The aromatic ring system of these compounds is able to include lysine and arginine side chains, supported by one or two phosphate groups that are attached to the half-moon-shaped molecule. Furthermore, we solved crystal structures of two different tweezer variants in complex with the enzyme Δ1-Pyrroline-5-carboxyl-dehydrogenase (P5CDH) and found that the tweezers are bound to a lysine and methionine side chain, respectively. Therefore, P5CDH was chosen as a target for the systematic analysis of co-crystallization with two different tweezer molecules, the diphosphate tweezer CLR01, which was also used for the 14-3-3 structures, and a monophosphate tweezer, where one phosphate group is replaced by a sterically less-demanding hydroxyl group. In both crystals, only one tweezer molecule is seen in the asymmetric unit despite the presence of two and four monomers of P5CDH, respectively, revealing an asymmetric binding mode of the tweezer to P5CDH, depending on the non-equivalent environment of the tweezer binding sites in the monomers.

P5CDH crystallizes as a tetramer consisting of a dimer of the physiologically relevant dimers with the N-termini of all four molecules in the asymmetric unit packing together in a large cleft between the two dimers formed by chains A and B, or C and D, respectively. Surprisingly, the CLR01 molecule was found in only one copy per tetramer in the asymmetric unit, and instead of binding to a lysine or arginine side chain, as expected, the Met17 of chain A—which actually belongs to artificially introduced linker residues —was seen as the guest inside the aromatic ring. The tweezer bound to monomer A is stabilized by packing against residues of monomer D. Interestingly, the regions around Met17 in monomers B, C, and D are disordered, indicating that the binding of CLR01 has a stabilizing effect on the N-terminus of monomer A, similar to the effect on the binding of a peptide to 14-3-3 described in the previous section. To further validate this binding mode, the anomalous signal of phosphorous and sulfur was measured at a wavelength of 1.698 Å at the synchrotron. Three peaks are observed at 2I/σI, at both phosphate groups of the tweezer and inside the ring system at a position corresponding to the sulfur atom of methionine 17. Although the anomalous signal is relatively weak, this strongly supports the binding mode of the tweezer encircling the Met17 side chain. A more detailed analysis of the tweezer binding modes using the CCP4 PISA software revealed that the largest hydrophobic Van der Waals interactions between the CLR01 and P5CDH monomer A are from the Met17 side chain bound inside the aromatic ring system, which is additionally clamped between two lysine residues that provide the positive charges to the region around the methionine. The interface of CLR01 to monomer A buries 487 Å2 of the solvent-excluded surface and covers about 69% of the tweezer’s surface.

>MGSSHHHHHHSSGLVPRGSHMTGAGLRWKHTSSLKVANEPVLAFTQGSPERDALQKALKDLKGRMEAIPCVVGDEEVWTSDVQYQVSPFNHGHKVAKFCYADKSLLNKAIEAALAARKEWDLKPIADRAQIFLKAADMLSGPRRAEILAKTMVGQGKTVIQAEIDAAAELIDFFRFNAKYAVELEGQQPISVPPSTNSTVYRGLEGFVAAISPFNFTAIGGNLAGAPALMGNVVLWKPSDTAMLASYAVYRILREAGLPPNIIQFVPADGPLFGDTVTSSEHLCGINFTGSVPTFKHLWKQVAQNLDRFHTFPRLAGECGGKNFHFVHRSADVESVVSGTLRSAFEYGGQKCSACSRLYVPHSLWPQIKGRLLEEHSRIKVGDPAEDFGTFFSAVIDAKSFARIKKWLEHARSSPSLTILAGGKCDDSVGYFVEPCIVESKDPQEPIMKEEIFGPVLSVYVYPDDKYKETLQLVDSTTSYGLTGAVFSQDKDVVQEATKVLRNAAGNFYINDKSTGSIVGQQPFGGARASGTNDKPGGPHYILRWTSPQVIKETHKPLGDWSYAYMQ[4x]>SDQDYRARLVYPFSGAISPHADIVDQATLAWAAMFGLLTDSLRHKSRRLQYGLLAARAYPRADREMLQIAADWIAWLFFMDDQCDETGIGRDLQRMIALHERFLAILDGATPEAHDCALTYALADLRRRLALRAPDNWLRRFSEHVRLYFTANRWETVNRQRGATPNVATYCAARLFSGAVYACFDLIELAEQIELPFYARHHSIVQQLEQAANNI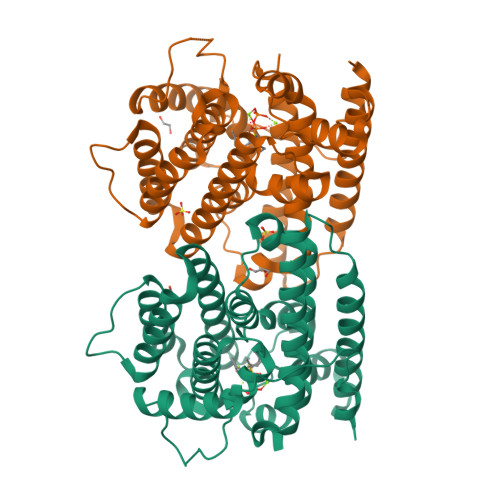ICWCNDVLSYPKEMQHGDRHNLVLVIQGEHQCSLPEAIDRALDLHAREVATFVRKRTCVPYFDAAVNTALEKYVTGLQFWICANRDWSLTATRYA[2x]Collagen's structure involves the assembly of three polyproline II helices, with each individual chain consisting of a three residue repeat sequence with the general form (Glycine–Xaa–Yaa). Within collagen's trademark triple-helical structure, three polyproline II helices are stitched together by a network of interstrand hydrogen bonding along the central axis of the right-handed triple helix. The triple helix is stabilized by the backbone NH groups of the Gly residues acting as hydrogen bond donors to the carbonyl oxygen of Xaa position residues in neighboring chains. To gain atomic level insight into these new rules we present two high-resolution crystal structures of collagen triple helices, with the first peptoid-containing collagen peptide structure.

We solved the structure of CMP 24, bearing the Xaa position Val residue, with the sequence [H–(POG)2(PRG)(POG)2(VOG)(POG)2(BrF–OG)(POG)–NH2] to 1.25 Å resolution. For one CMP we included a 4-bromophenylalanine (BrF) residue for phasing using single-wavelength anomalous diffraction, but molecular replacement was successful for both structures. In the structure with the Xaa position Val residue, a void is present along the surface of the triple helix at the site of Val incorporation. This is a result of Val's secondary backbone amine being sterically unencumbered compared to the tertiary backbone amine of N-substituted residues like Pro, Hyp, or peptoids. The consequence of this hole is solvent exposure, clearly indicated the presence of a water molecule next to the Val residues in our structure. This water molecule is well-positioned to hydrogen bond with the NH group of the Val residue at approximately 3.0 Å away. Importantly, this water is also positioned in close proximity with the Cα of the Gly residue adjacent to the Xaa Val approximately 3.3 Å away. This Gly Cα corresponds to the azGly substitution site in our model system. In addition, we have reported two new collagen crystal structures, with the first structure of a collagen triple helix containing a peptoid residue. These structures, containing either a Val or NmetG residue in the Xaa position and reveal how the NmetG residues protect the collagen backbone from solvent while the Val residues expose it.

>[3x]PPGPPGPRGPPGPPGVPGPPGPPGYPGPPGX N-(7-fluoro-2,3-dioxo-6-(trifluoromethyl)-3,4-dihydroquinoxalin-1(2H)-yl)-2-hydroxybenzamide | C16 H9 F4 N3 O4 | 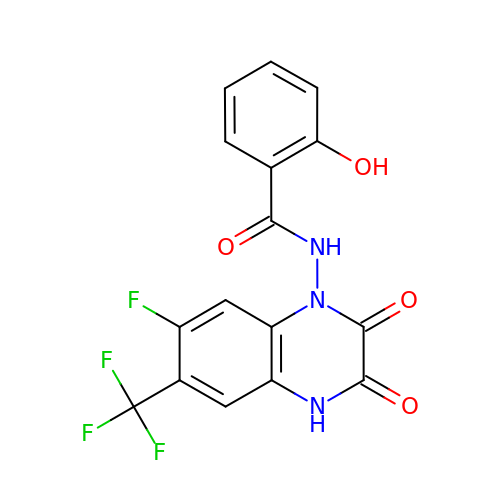MCKOVZZCGOMMIB-UHFFFAOYSA-N> MYEAIGHRVEDGVAEITIKLPRHRNALSVKAMQEVTDALNRAEEDDSVGAVMITGAEDAFCAGFYLREIPLDKGVAGVRDHFRIAALWWHQMIHKIIRVKRPVLAAINGVAAGGGLGISLASDMAICADSAKFVCAWHTIGIGNDTATSYSLARI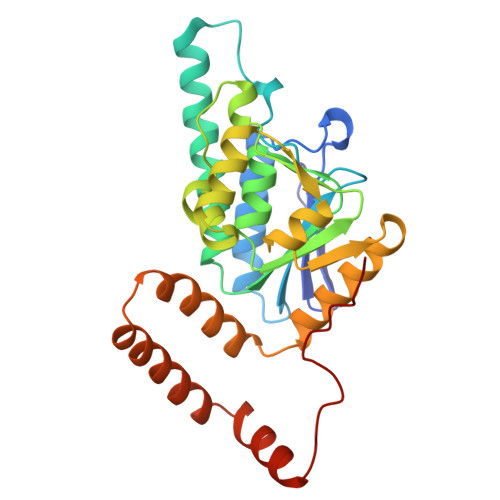VGMRRAMELMLTDRTLYPEEAKDWGLVSRVYPKDEFREVAWKVARELAAAPTHLQVMAKERFHAGWMQPVEECTEFEIQNVIASVTHPHFMPCLTRFLDGHRADRPQVELPAGV> MLCQQMIRTTAKRSSNIMTRPIIMKRSVHFKDGVYENIPFKVKGRKT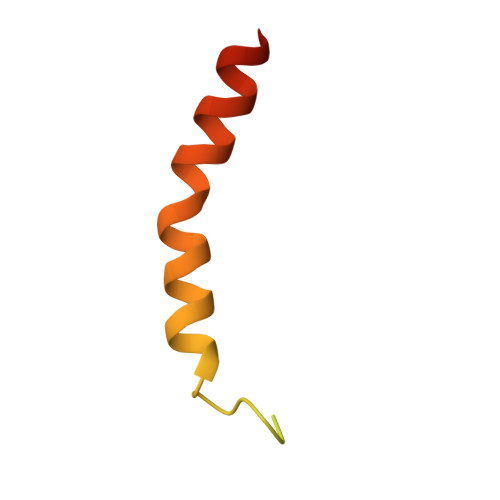PYALSHFGFFAIGFAVPFVACYVQLKKSGAF> MGSDKIHHHHHHVGKVADTLKPGDRVLLSFEDESEFLVDLEKDKKLHTHLGIIDLNEVFEKGPGEIIRTSAGKKGYILIPSLIDEIMNMKRRTQIVYPKDSSFIAMMLDVKEGDRIIDTGVGSGAMCAVLARAVGSSGKVFAYEKREEFAKLAESNLTKWGLIER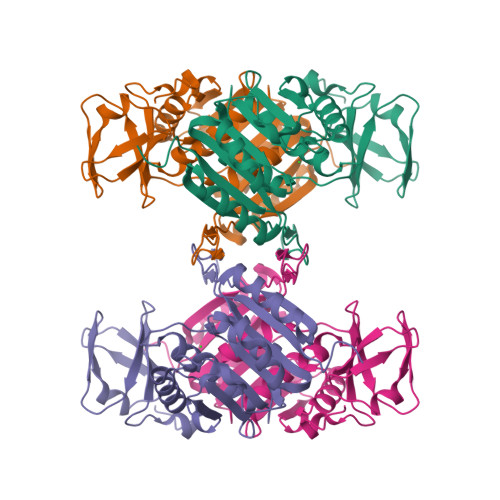VTIKVRDISEGFDEKDVDALFLDVPDPWNYIDKCWEALKGGGRFATVCPTTNQVQETLKKLQELPFIRIEVWESLFRPYKPVPERLRPVDRMVAHTAYMIFATKVCRREETE> SMKDYDELLKYYELHETIGTGGFAKVKLACHILTGEMVAIKIMDKNTLGSDLPRIKTEIEALKNLRHQHICQLYHVLE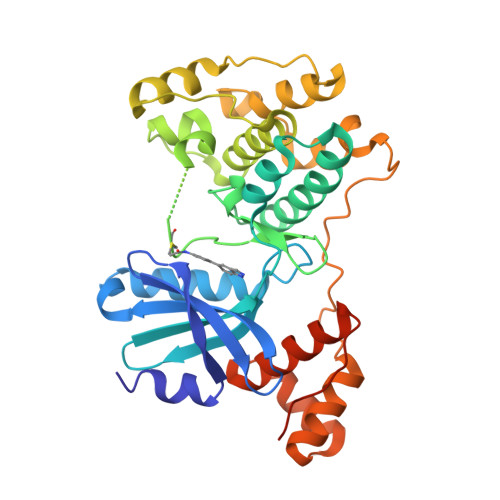TANKIFMVLEYCPGGELFDYIISQDRLSEEETRVVFRQIVSAVAYVHSQGYAHRDLKPENLLFDEYHKLKLIDFGLCAKPKGNKDYHLQTCCGSLAYAAPELIQGKSYLGSEADVWSMGILLYVLMCGFLPFDDDNVMALYKKIMRGKYDVPKWLSPSSILLLQQMLQVDPKKRISMKNLLNHPWIMQDYNYPVEWQSKNPFIHLDDDCVTELSVHHRNNRQTMEDLISLWQYDHLTATYLLLLAKKARGKPVRLRLSSFSCGQASATPFT>[2x]MAKKTKQRRPMGFPPGPPGLPFIGNIYSLAASSELPHVYMRKQSQVYGEIFSLDLGGISTVVLNGYDVVKECLVHQSEIFADRPCLPLFMKMTKMGGLLNSRYGRGWVDHRRLAVNSFRYFGYGQKSFESK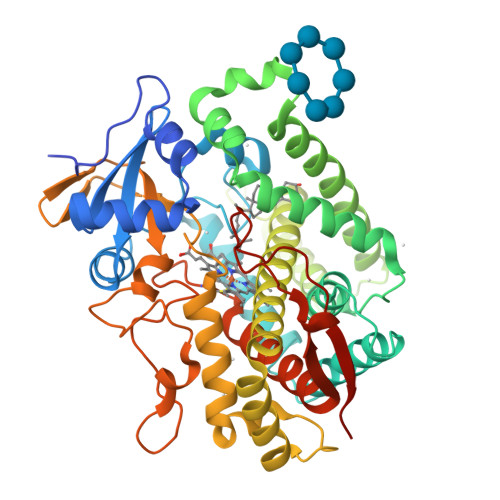ILEETKFFNDAIETYKGRPFDFKQLITNAVSNITNLIIFGERFTYEDTDFQHMIELFSENVELAASASVFLYNAFPWIGILPFGKHQQLFRNAAVVYDFLSRLIEKASVNRKPQLPQHFVDAYLDEMDQGKNDPSSTFSKENLIFSVGELIIAGTETTTNVLRWAILFMALYPNIQGQVQKEIDLIMGPNGKPSWDDKCKMPYTEAVLHEVLRFCNIVPLGIFHATSEDAVVRGYSIPKGTTVITNLYSVHFDEKYWRDPEVFHPERFLDSSGYFAKKEALVPFSLGRRHCLGEHLARMEMFLFFTALLQRFHLHFPHELVPDLKPRLGMTLQPQPYLICAERRHHHHHH(4R)-3-{(2S,3S)-2-hydroxy-3-[(3-hydroxy-2-methylbenzoyl)amino]-4-phenylbutanoyl}-5,5-dimethyl-N-(2-methylbenzyl)-1,3-thiazolidine-4-carboxamide 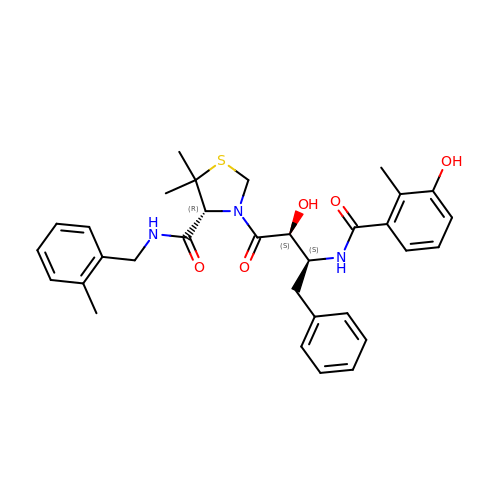| C32 H37 N3 O5 S | CUFQBQOBLVLKRF-RZDMPUFOSA-N> GHMRVEIWSDIACPWCYVGKARFEKALAAFPHRDGVEVVHRSFELDPGRAKDDVQPVLTMLTAKYGMSQEQAQAGEDNLGAQAAAEGLAYRTRDRDHGSTFDLHRLLHLAKERGRHEALLDAFYRGNFADERSVFNDDERLVELAVGAGLDAEEVRAVLADPAAYADEVRADEREAAQLGATGVPFFV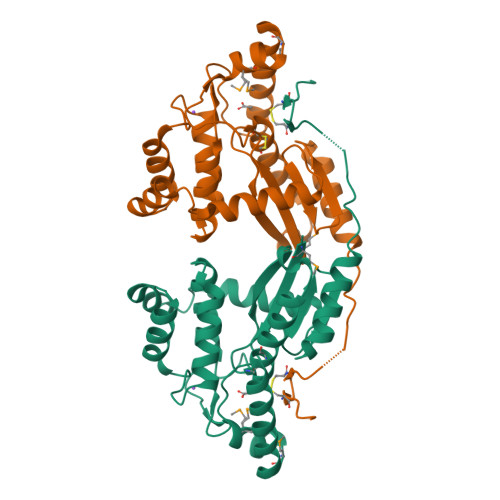LDRAYGVSGAQPAEVFTQALTQAWGERTPLKLIDDGGAEACGPDGCAVPGH> MATTCRTADGDMLDSLCYHVYGHLLG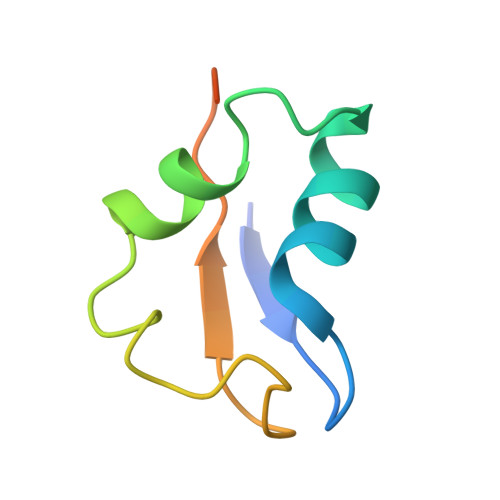CVEATLDANPGLADEQQPFRAGLLISFPDMPVVNVEQVRLWD Dissociation of U1 snRNP is thought to be triggered by the DEAD-box protein Prp28 (4,5), acting to disrupt the short U1:5′ splice site RNA duplex or remodel protein–RNA contacts at the 5′ splice site (or both). The 588-aa Prp28 polypeptide is a member of the DEAD-box family and includes the 12 conserved amino acid sequence motifs that define this clade of nucleic acid-dependent NTP phosphohydrolases. In the present study, we demonstrate that yeast Prp28 is a bona fide RNA-dependent ATPase, albeit with a low turnover number. Prp28 comprises two structural domains (referred to as RecA-like) that are splayed widely apart.

We report the crystal structure of a truncated ATPase-active Prp28-(127–588) protein in a complex with AMPPNP and magnesium that exemplifies a wide-open domain arrangement that is not poised for ATP hydrolysis. We grew crystals from a mixture of SeMet-substituted Prp28-(127–588), AMPPNP, MgCl2 and 10-mer RNA oligonucleotide. The crystals were in space group P3221 with two Prp28 protomers per asymmetric unit. The maps revealed Fo–Fc density for AMPPNP•Mg2+ in the active site of the B protomer, but there was no electron density corresponding to the RNA. The C domains differ by virtue of a large rigid body motion around an interdomain linker segment, 402GVETSEP409 that results in a 45 Å displacement of the Cα atom of the Asn577 residue (located at the end of the C-terminal α helix). We conclude that Prp28 can sample a broad range of domain orientations in the absence of a bound RNA and/or interactions with the spliceosome. The nucleotide was bound wholly within the N domain. The adenine nucleobase, in anti conformation with respect to the ribose, is sandwiched between Phe194, on which it makes a π stack, and Thr198 Cγ, which makes van der Waals contact to the adenine N6, C5, C6 and N7 atoms. The eponymous Gln201 of the Q motif makes hydrogen bonds with the adenine N6 and N7 atoms that we presume confer adenine specificity. The wide-open domain conformation we see in the absence of a bound RNA suggests that RNA engagement is needed in order to trigger domain closure and capture of the triphosphate•Mg2+ complex in a productive orientation by motif VI of the C domain.

>SNAAESSYMGKHWTEKSLHEMNERDWRILKEDYAIVTKGGTVENPLRNWEELNIIPRDLLRVIIQELRFPSPTPIQRITIPNVCNMKQYRDFLGVASTGSGKTLAFVIPILIKMSRSPPRPPSLKIIDGPKALILAPTRELVQQIQKETQKVTKIWSKESNYDCKVISIVGGHSLEEISFSLSEGCDILVATPGRLIDSLENHLLVMKQVETLVLDEADKMIDLGFEDQVTNILTKVDINADSAVNRQTLMFTATMTPVIEKIAAGYMQKPVYATIGVETGSEPLIQQVVEYADNDEDKFKKLKPIVAKYDPPIIIFINYKQTADWLAEKFQKETNMKVTILHGSKSQEQREHSLQLFRTNKVQIMIATNVAARGLDIPNVSLVVNFQISKKMDDYIHRIGRTGRAANEGTAVSFVSAAEDESLIRELYKYVRKHDPLNSNIFSEAVKNKYNVGKQLSNEIIY[2x]>[2x]MMKPEDVIKEQCARAKVVAELWHGFTGGAPKAALENLVVEFNKAQQGRCVRPVPQGGYRDLSTKIKAAFAAGKVPTMAQAFENNIALYLEAKALLPIE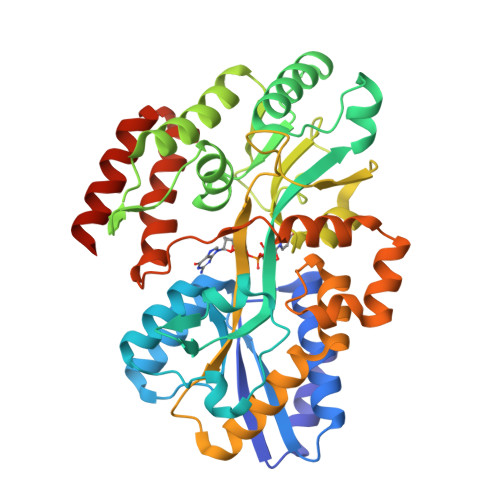SLGVKLQGVNLTFLNAVRFGGVVYGVPFNKSIQVLYYNKDLLKKHGVPVPATLEEFVAAAKKLSRAEGGPVYWFQPDASTFAYFFFNLGGSYLKDGKLVLNSKEAVEALTLLQNGVKEGWAKPITSGYINQNLGSGPYAFSVDTSAGYTAYLRAAKFDLGVATLPGRTKGQPGYGLVQGTNLVVFRQASKEEQAVAKDFLEFVLSPRAQAVFATATGYVPVTEGALKDPVYQAYAAENPDYATIVRQSRYAKFEPALAEWEQIRFDILGQAIKEAILNKADPKAALDRAQKLAEDLLSSRTRHHHHHH3-({4-[(1E)-3-morpholin-4-yl-3-oxoprop-1-en-1-yl]-2,3-bis(trifluoromethyl)phenyl}sulfanyl)aniline | C21 H18 F6 N2 O2 S | 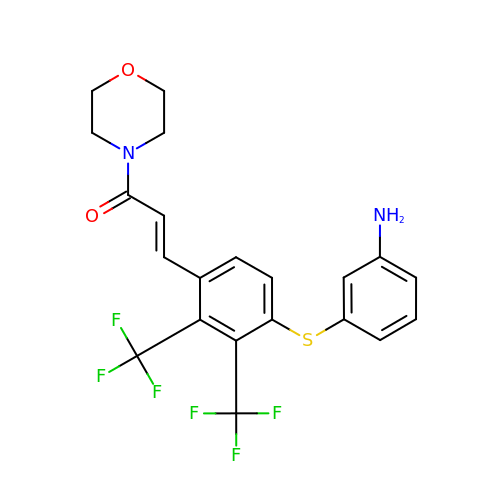KLSZVPNVFKKIRD-FNORWQNLSA-N> MSQEQGKIYIVEDDMTIVSLLKDHLSASYHVSSVSNFRDVKQEIIAFQPDLILMDITLPYFNGFYWTAELRKFLTIPIIFISSSNDEMDMVMALNMGGDDFISKPFSLAVLDAKLTAILRRSQQFIQQELTFGGFTLTREGLLSSQDKEVILSPTENKILSILLMHPKQVVSKESLLEKLWENDSFIDQNTLNVNMTRLRKKIVPIGFDYIHTVRGVGYLLQDPNSSSVDKLAAALEHHHHHH;> MSQEQGKIYIVEDDMTIVSLLKDHLSASYHVSSVSNFRDVKQEIIAFQPDLILMDITLPYFNGFYWTAELRKFLTIPIIFISSSNDEMDMVMALNMGGDDFISKPFSLAVLDAKLTAILRRSQQFIQQELTFGGFTLTREGLLSSQDKEVILSPTENKILSILLMHPKQVVSKESLLEKLWENDSFIDQNTLNVNMTRLRKKIVPIGFDYIHTVRGVGYLLQNDPSSSVDKLAAALEHHHHHH

Here, we describe the crystal structures of the N-terminal RD and the C-terminal ED of the lantibiotic resistance-associated RR NsrR from S. agalactiae. NsrR is part of the nisin resistance operon. The expression of the genes of this operon is induced by a TCS consisting of the HK NsrK and the RR NsrR. NsrR belongs to the OmpR/PhoB family of RRs.

The structure of NsrR-ED from S. agalactiae was determined using experimental phases from a single-wavelength anomalous dispersion dataset from the rectangular plate-shaped crystal derivatized with platinum at a resolution of 1.6 Å in space group P21212. The asymmetric unit contains two copies of NsrR-ED related by two-fold rotational symmetry. The ED domain of NsrR consists of six β-strands and three α-helices in a β6-β7-β8-β9-α6-α7-α8-β10-β11 topology (the secondary structure elements are counted in continuation of those of the RD). The effector domain starts with a 4-stranded antiparallel β-sheet, followed by three α-helices and eventually ends in a C-terminal β-hairpin. The structure of NsrR-ED also contains such a wHTH motif built up by helices α7 and α8. In the structure of NsrR-ED, helix α8 is identified as the recognition helix, α7 as the positioning helix, and the loop region between helices α7-α8 as transactivation loop as observed in other RRs. The 16-residue long, solvent-exposed recognition helix α8 of NsrR-ED contains four positively charged residues that can potentially interact with DNA. These are Arg198, Arg200, Lys201, and Lys202. The rmsd between the three helices of the effector domain (including the two helices forming the wHTH motif) of PhoB and NsrR-ED is 1.6 Å over 47 Cα atoms, clearly indicating that NsrR belongs to the OmpR/PhoB family of RRs. As a result, a highly positive groove is created by the two ED domains of NsrR which likely represents the DNA binding site as observed in KdpE.>LKCNKLIPLAYKTCPAGKNLCYKMFMVSNKTVPVKRGCIDVCPK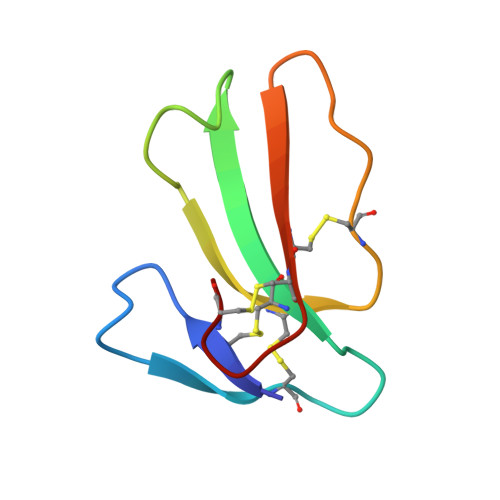NSLLVKYVCCNTDRCN[6x]>MIAGSMVALVTPFDAQGRLDWDSLAKLVDFHLQDGTNAIVAVGTTGESATLDVEEHIQVVRRVVDQVKGRIPVIAGTGAN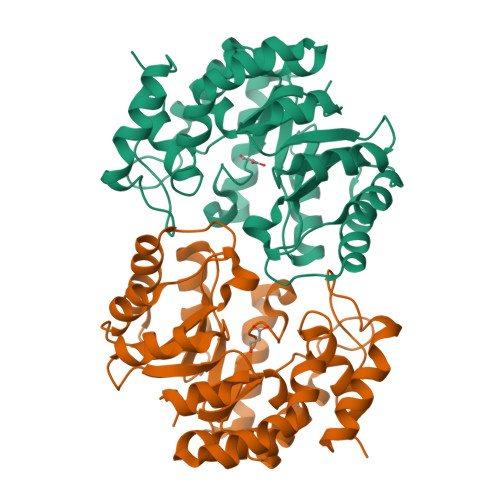STREAVALTEAAKSGGADACLLVTPYYNKPTQEGMYQHFRHIAEAVAIPQILYNVPGRTSCDMLPETVERLSKVPNIIGIKEATGDLQRAKEVIERVGKDFLVYSGDDATAVELMLLGGKGNISVTANVAPRAMSDLCAAAMRGDAAAARAINDRLMPLHKALFIESNPIPVKWALHEMGLIPEGIRLPLTWLSPHCHDPLRQAMRQTGVLA[2x]> KQFTKCELSQLLKDIDGYGGIAL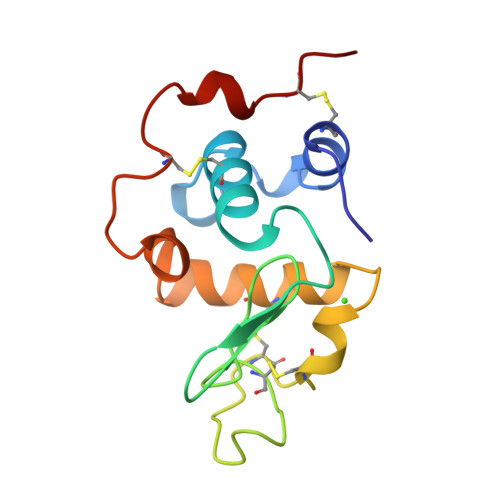PELICTMFHTSGYDTQAIVENDESTEYGLFQISNKLWCKSSQVPQSRNICDISCDKFLDDDITDDIMCAKKILDIKGIDYWLAHKALCTEKLEQWLCEKL>MSLDQETVGNVVLLAIV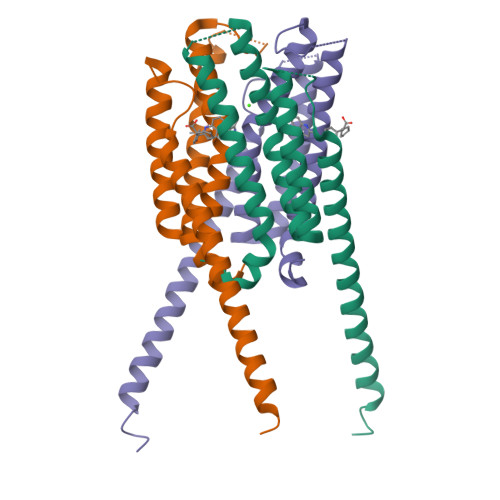TLISVVQNGFFAHKVEHESRTQNGRSFQRTGTLAFERVYTANQNCVDAYPTFLAVLWSAGLLCSQVPAAFAGLMYLFVRQKYFVGYLGERTQSTPGYIFGKRIILFLFLMSVAGIFNYYLIFFFGSDFENYIATISTTISPLLLIPEGHHHHHH[6x]> MTNRLELSGIICRTPLRKVSPSGIPHCQFVLEHRS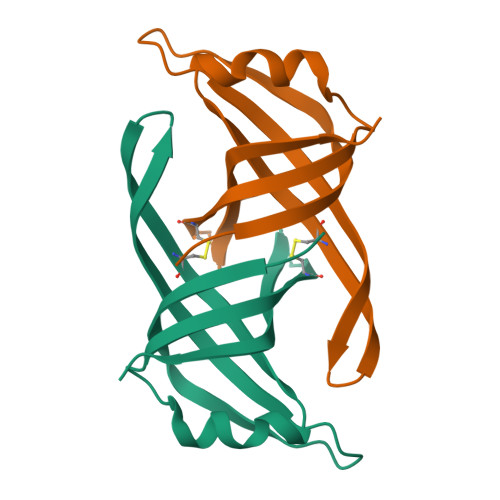VQEEAGFHRQAWCQMPVIISGHENQAITHSITVGSAVTVRGFISCHKAKNGLSKMVLHAEQIELIDSGDLEHHHHHH> MSNIFLELQDGDKTVYTHTSLIEESKQEQIQAIYDKVPQWTNGGRFLGFWLSMEAVNRVQSVAKLPIYYRAGIVATSTLLGGLVSSLVFWKSGNENQVAKLANGAPVYLKKWEVPELSKLYFFLDDDNNF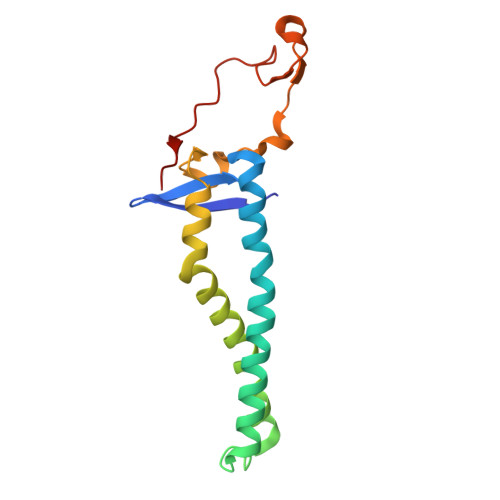KPSLNHHAVTQGRQYYKIYQHN>MLQLWSKFDVGDWLESIHLGEHRDRFEDHEIEGAHLPALTKEDFVELGVTRVGHRENIERALRQLDGSRRHHHHHH[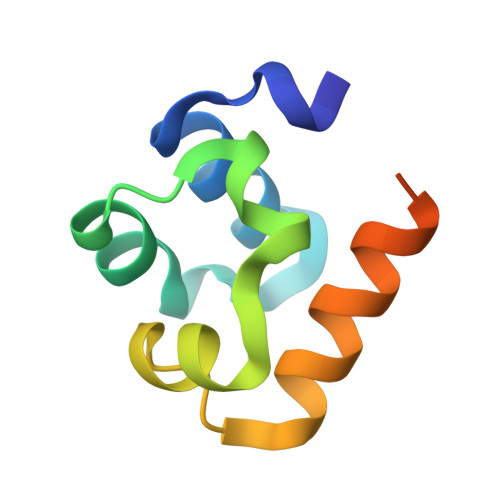3x]>MVLIFHGKPVHGAIFAMDGTMFDTERLRFQTLQQASQELIGQEFSHEYLMQCLGLSATTAEKLAQRLYGVDVPYKEIRKRADEMELEHIRKHGVPIKKGLVQVLERLRKSGLRMAVATSSRRAIAEEYLINANVYKFFDVITCGDEVEQGKPHPEIFLKAASQLHLDANQCLMFEDSENGLTSAHTSKGLTILLKDIKEPNDEMLEKAHFYYDQMYDFLTDLDQFIPVMDMPEMQEPFPQSLNQLTVGIHGFGAIGGGYIAQILSHWDGYTKPKRIIASTRNSLFREAVNAFGTYSIRYGQFSYDERIENMSIVDSDNEQQMLEMYTHSSLIALCLPEQAIESESKIIAKGLYARFNSQLETCIEPL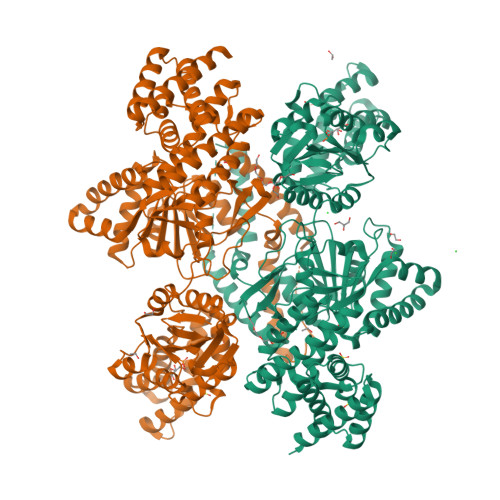TFLIILNKVGAKYLVMKHLKEALLELTNDEDVTEHILKEHYFCDTVVNRMVSKLSNQNLYRQLRIKHNFLEQHLEDVEQEDQIEIEDCNKLTPDQLNQASIYVDNMRRNFQPGHILQSMDLILFHSETDMPIYVEKGSPLLEKLRQVVLVDQITDIQLIKNRLWNGVHAMLAWYASLMGYESIGVAMGDHLVKAFAENLIAEVKQGLAIVLPNYAKDLDRMSQSFLDSCEYAFKDPCQRVARDPLRKLNHNERVMASIAVNIRHDLPYKNLLKGAALGYAYAIQFLEIEETKAVEHLQQQIQNLDLSTAQRRQLEAELVQLIQYLFSEQGKQPLDIKSNNTKTTSTQYVAAALEHHHHHH[4x]>HHHHHHGSDPIHYDKITEEINKAIDDAIAAIEQSET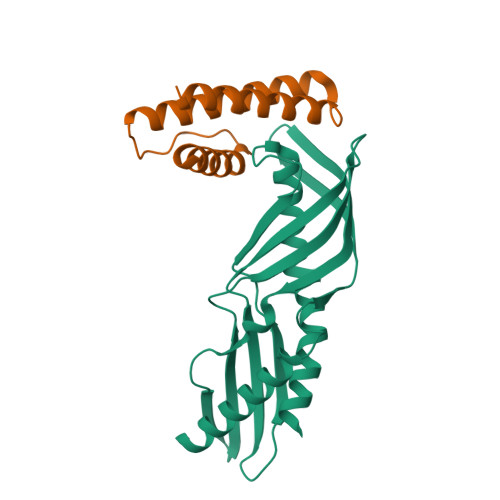IDPMKVPDHADKFERHVGILDFKGELAMRNIEARGLKQMKRQGDANVKGEEGIVKAHLLIGVHDDIVSMEYDLAYKLGDLHPTTHVISDIQDFVVALSLEIPDEGNITMTSFEVRQFANVVNHIGGLSILDPIFGVLSDVLTAIFQDTVRKEMTKVLAPAFKRELEKN[3x];>HHHHHHGSSPKEEKFKKKLEEELKKIRERLLMVFDEERVEEYMKIMKEVIEKILENRKKGSKEKVEIPPGMEWFYENFLRYYDYEEEKLEKEEKE[3x]>MEHHHHHHATNLRGVMAALLTPFDQQQALDKASLRRLVQFNIQQGIDGLYVGGSTGEAFVQSLSEREQVLEIVAEEAKGKIKLIAHVGCVSTAESQQLAASAKRYGFDAVSAVTPFYYPFSFEEHCDHYRAIIDSADGLPMVVYNIPALSGVKLTLDQINTLVTLPGVGALKQTSGDLYQMEQIRREHPDLVLYNGYDNIFASGLLAGADGGIGSTYNIMGWRYQGIVKALKEGDIQTAQKLQTECNKVIDLLIKTGVFRGLKTVLHYMDVVSVPLCRKPFGPVDEKYLPELKALAQQLMQERG[4x]

N-Acetylneuraminic acid lyase (NAL; EC 4.1.3.3, otherwise known as N-acetylneuraminic acid aldolase or sialic acid aldolase) catalyzes the reversible aldol condensation of N-acetylmannosamine (ManNAc) with pyruvate to yield the most abundant sialic acid N-acetylneuraminic acid (Neu5Ac). Sialic acids are essential components of complex carbohydrates that play pivotal roles as recognition signals in a variety of biological processes. The residue responsible for this alteration of specificity at position 192 lies at one end of the active-site cleft opposite the active-site catalytic residue Lys165, which forms a Schiff base with the substrate as part of the catalytic cycle. In order to probe the mechanism by which alteration of the residue at position 192 affects substrate specificity, we have undertaken an analysis of the activity of all 20 variants of NAL at position 192 along with an X-ray structural analysis of the E192N enzyme in the absence and in the presence of a competitive inhibitor, (2R,3R)-2,3,4-trihydroxy-N,N-dipropylbutanamide (THB).

We therefore identified new conditions for the crystallization of E. coli NAL (in space group P21) that avoided the use of sulfate ions and allowed us to solve the structures of both the wild type and the E192N variant in the presence and in the absence of a number of ligands. The crystal structures of wild-type E. coli NAL and the E192N variant were solved at 2.2 Å and 1.8 Å, respectively, and show a tertiary structure identical to that previously observed. The overall RMSD between the Cα atoms in the wild-type structure and the Cα atoms in the E192N structure is 0.3 Å. The only significant differences are the orientation of Asn192 compared to that of the wild-type Glu192 and the resulting changes in surface potential at the entrance of the catalytic pocket when the negatively charged glutamate is replaced. In contrast, in the E192N variant, the amide of Asn192 points out of the active-site cleft (a position disfavored for glutamate due to unfavorable contacts with the neighboring hydrophobic residues Tyr172 and Ile243), and this conformation produces a larger hydrophobic binding surface that is ideal for interaction with THB. An asparagine at position 192, on the other hand, provides an uncharged surface with no steric interference with DPAH binding.> X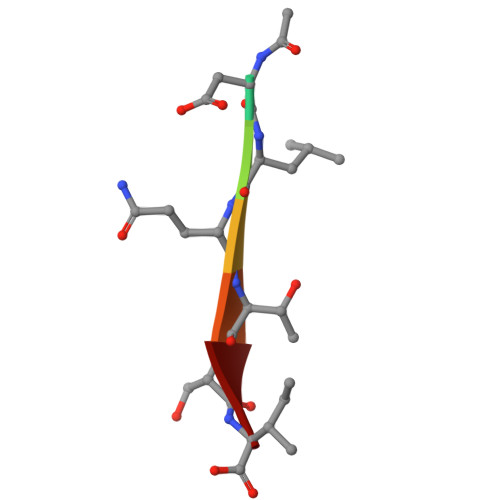DLQTSI> METSDIQIFYQEDPECQNLSENSCPPSEVSDTNLYSPFKPRNYQLELALPAMKGKNTIICAPTGCGKTFVSLLICEHHLKKFPQGQKGKVVFFANQIPVYEQQKSVFSKYFERHGYRVTGISGATAENVPVEQIVENNDIIIL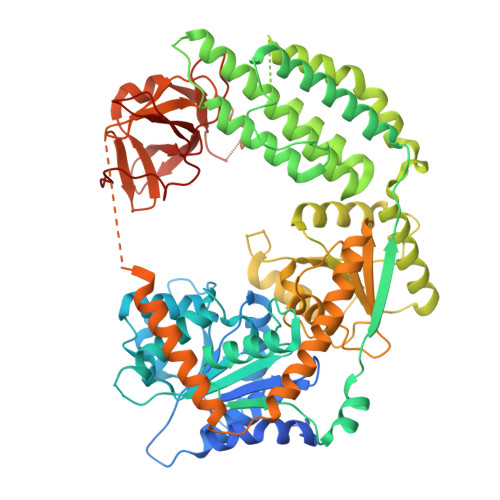TPQILVNNLKKGTIPSLSIFTLMIFDECHNTSKQHPYNMIMFNYLDQKLGGSSGPLPQVIGLTASVGVGDAKNTDEALDYICKLCASLDASVIATVKHNLEELEQVVYKPQKFFRKVESRISDKFKYIIAQLMRDTESLAKRICKDLENLSQIQNREFGTQKYEQWIVTVQKACMVFQMPDKDEESRICKALFLYTSHLRKYNDALIISEHARMKDALDYLKDFFSNVRAAGFDEIEQDLTQRFEEKLQELESVSRDPSNENPKLEDLCFILQEEYHLNPETITILFVKTRALVDALKNWIEGNPKLSFLKPGILTGRGKTNQNTGMTLPAQKCILDAFKASGDHNILIATSVADEGIDIAQCNLVILYEYVGNVIKMIQTRGRGRARGSKCFLLTSNAGVIEKEQINMYKEKMMNDSILRLQTWDEAVFREKILHIQTHEKFIRDSQEKPKPVPDKENKKLLCRKCKALACYTADVRVIEECHYTVLGDAFKECFVSRPHPKPKQFSSFEKRAKIFCARQNCSHDWGIHVKYKTFEIPVIKIESFVVEDIATGVQTLYSKWKDFHFEKIPFDPAEMSK>MKVYITYGTADFLKTIVKKHPSENILLMQGQENAILIHETSGDTVFQAPHAYEVIDQVGEIKHPGFAVLANIAVTQEGRPLFENKFKNRAGKVENEPGFEAIRVLRPLDSDTYVILTLWETERAFQDWQQSDSYKEAHKKR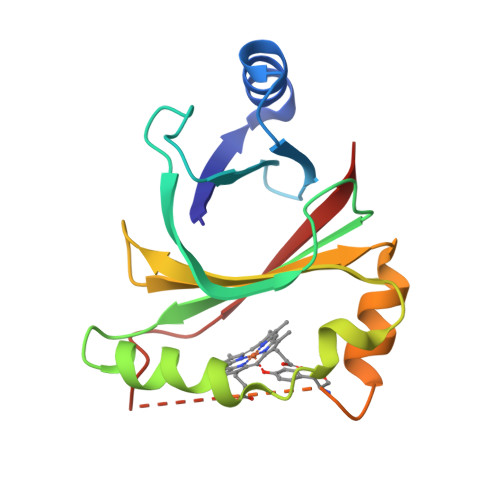GTSAGIDTTSIFSRPSYVTTYFAVE[6x]> MAHHHHHHMNPLLISSGEPAGIGPDLCLALAETDLPVVILGDLSLLEARASELNLSIKFLEYSPHQSFKKKAGYLTVWPVPCAAPVISGELNPQNAAYVMELLTLGASLCSKGEFSALVTAPVHKANINAA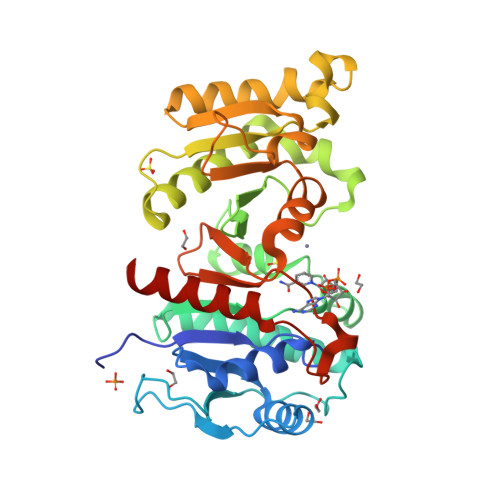GITFTGHTEFFADFFEVETVVMMLACSQMKVALVTTHLPLRMVPDAISSLLIIKVIQQLHHSLKHDFGIQSPKINVAGLNPHAGESGYLGREEIEIITPALNTLKNQGIDVLGPLPADTMFITNHINHCDAYVAMYHDQGLPVLKYAGFNEAVNITLGLPIIRTSVDHGTALELAGKNKANPGSMLAAVKMAKDMALTRIK>DRRHVLLQAEFYQRSEGPDKAWAQFGFHFDADELFHVELDAAQTVWRLPEFGRFASFEAQGALQNMAVGKQNLEVMISNSNRSQQDFVTPELALFPAEAVSLEEPNVLICYADKFWPPVATMEWRRNGAVVSEGVYDSVYYGRPDLLFRKFSYLPFVPQRGDVYSCAVRHWGAEGPVQRMWEPEVPEPPSE[3x];>[3x]DRPAVVHSVRALMLAERQGGGGSGGGGSGGGGSFFYGKIGECHYLNGTERVRFLDRQIYNRQQFAHFDSDVGKFVADTPLGE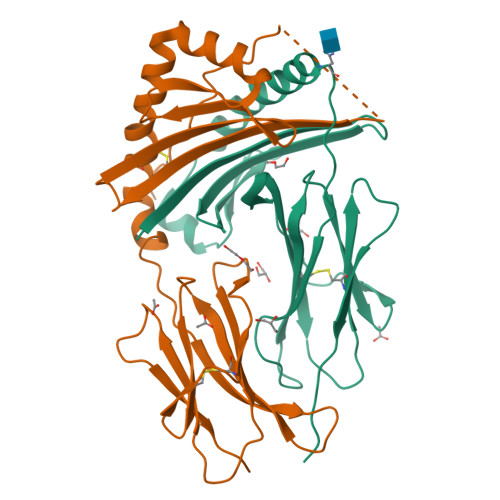PQAEYWNSNAELLENLMNEVDRVCRHNYGILESFTVQRSVEPKVRVSALQSGSLPETDRLACYVTGFYPPEIEVKWFLNGREETERVVSTDVMQNGDWTYQVLVVLETVPRRGDSYVCRVEHASLRQPISQAWEPPADAGRSK> SHNECISVKGRIYSILKQIGSGGSSKVFQVLNEKKQIYAIKYVNLEEADNQTLDSYRNEIAYLNKLQQHSDKIIRLYDYEITDQYIYMVMECGNIDLNSWLKKKKSIDPWERKSYWKNM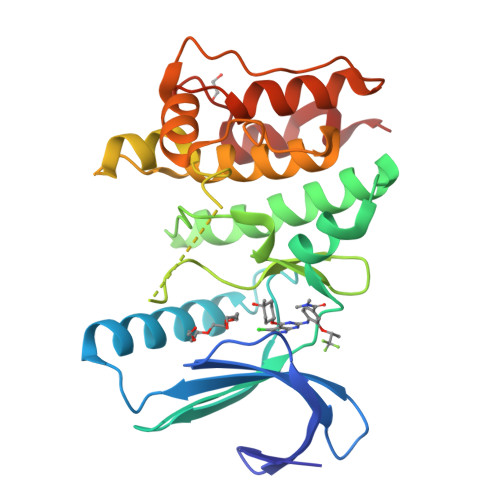LEAVHTIHQHGIVHSDLKPANFLIVDGMLKLIDFGIANQMQPDTTSVVKDSQVGTVNYMPPEAIKDMSSSRENGKSKSKISPKSDVWSLGCILYYMTYGKTPFQQIINQISKLHAIIDPNHEIEFPDIPEKDLQDVLKCCLKRDPKQRISIPELLAHPYVQIQTLE>[2x]DALKVNRAPVGVEPQEVHKWLQSFNWDFKENRTKYPTKYHMANETKEQFKVIAKEYARMEAAKDERQFGTLLDGLTRLGAGNKVHPRWGETMKVISNFLEVGEYNAIAASAMLWDSATAAEQKNGYLAQVLDEIRHTHQCAFINHYYSKHYHDPAGHNDARRTRAIGPLWKGMKRVFADGFISGDAVECSVNLQLVGEACFTNPLIVAVTEWASANGDEITPTVFLSVETDELRHMANGYQTVVSIANDPASAKFLNTDLNNAFWTQQKYFTPVLGYLFEYGSKFKVEPWVKTWNRWVYEDWGGIWIGRLGKYGVESPASLRDAKRDAYWAHHDLALAAYAMWPLGFARLALPDEEDQAWFEANYPGWADHYGKIFNEWKKLGYEDPKSGFIPYQWLLANGHDVYIDRVSQVPFIPSLAKGTGSLRVHEFNGKKHSLTDDWGERQWLIEPERYECHNVFEQYEGRELSEVIAEGHGVRSDGKTLIAQPHTRGDNLWTLEDIKRAGCVFPDPLAKF;>[2x]PQSSQVTKRGLTDPERAAIIAAAVPDHALDTQRKYHYFIQPRWKRLSEYEQLSCYAQPNPDWIAGGLDWGDWTQKFHGGRPSWGNEST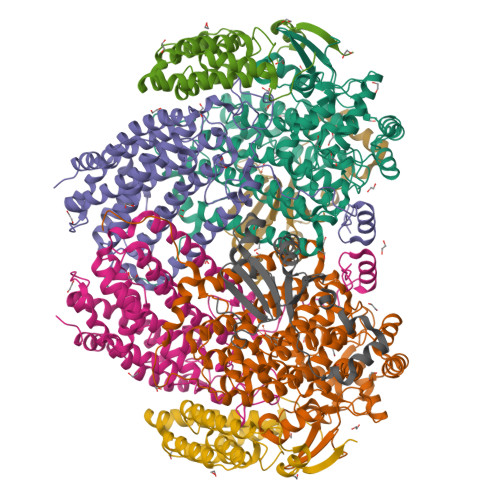ELRTTDWYRHRDPARRWHHPYVKDKSEEARYTQRFLAAYSSEGSIRTIDPYWRDEILNKYFGALLYSEYGLFNAHSSVGRDCLSDTIRQTAVFAALDKVDNAQMIQMERLFIAKLVPGFDASTDVPKKIWTTDPIYSGARATVQEIWQGVQDWNEILWAGHAVYDATFGQFARREFFQRLATVYGDTLTPFFTAQSQTYFQTTRGAIDDLFVYCLANDSEFGAHNRTFLNAWTEHYLASSVAALKDFVGLYAKVEKVAGATDRAGVSEALQRVFGDWKIDYADKIGFRVDVDQKVDAVLAGYKN;>[2x]AKREPIHDNSIRTEWEAKIAKLTSVDQATKFIQDFRLAYTSPFRKSYDIDVDYQYIERKIEEKLSVLKTEKLPVADLITKATTGEDAAAVEATWIAKIKAAKSKYEAERIHIEFRQLYKPPVLPVNVFLRTDAALGTVLMEIRNTDYYGTPLEGLRKERGVKVLHLQA;>[2x]SAHNAYNAGIMQKTGKAFADEFFAEENQVVAESNAVVLVLMKSDEIDAIIEDIVLKGGKAKNPSIVVEDKAGFWWIKADGAIEIDAAEAGELLGKPFSVYDLLINVSSTVGRAYTLGTKFTITSELMGLDRALTDI> MGSKSKVDNQFYSVEVGDSTFTVLKRYQNLKPIGSGAQGIVCAAYDAVLDRNVAIKKLSRPFQNQTHAKRAYRELVLMKCVNHKNIISLLNVFTPQKTLEEFQDVYLVMELMDANLCQVIQMELDHERMSYLLYQMLCGIKHLHSAGIIHRDLKPSNIVVKSDCTLKILDFGLARTAGTSFMMTPYVVTRYYRAPEVILGMGYKENVDIWSVGCIMGEMVRHKILFPGRDYIDQWNKVIEQLG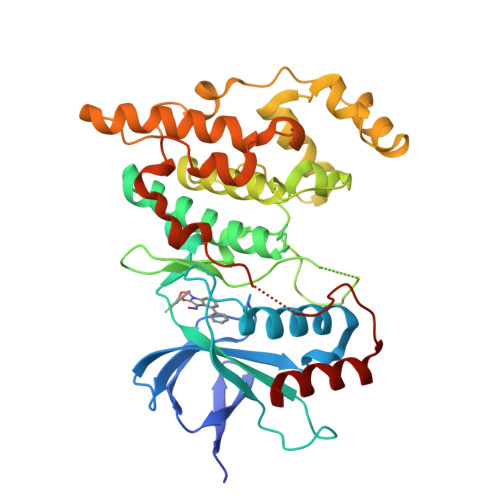TPCPEFMKKLQPTVRNYVENRPKYAGLTFPKLFPDSLFPADSEHNKLKASQARDLLSKMLVIDPAKRISVDDALQHPYINVWYDPAEVEAPPPQIYDKQLDEREHTIEEWKELIYKEVMNSE> DYKDDDDKSNVDPQHRLSQKLKERLGYLGVYYKRDTAFFFRRMSPADKRKLLDELRSIYRTIVLEYFNTDAKVN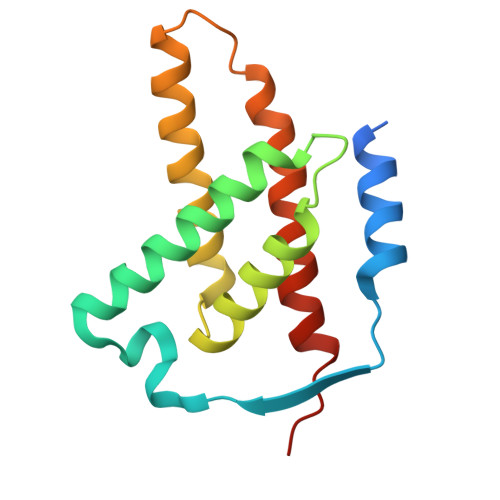ERIDEFVSKAFFADISVSQVLEIHVELMDTFSKQLKLEGRSEDILLDYRLTLIDVIAHLSEMYRRSIPREV>AFQETNPPAGPVRAIAEYERSAAVLVRYPFGIPMELIKELAKNDKVITIVASESQKNTVITQYTQSGVNLSNCDFIIAKTDSYWTRDYTGWFAMYDTNKVGLVDFIYNRPRPNDDEFPKYEAQYLGIEMFGMKLKQTGGNYMTDGYGSAVQSHIAYTENSSLSQAQVNQKMKDYLGITHHDVVQDPNNTYIDHVDCWGKYLAPNKILIRKVPDNHPQHQALEDMAAYFAAQTCAWGTKYEVYRALATNEQPYTNSLILNNRVFVPVNGPASVDNDALNVYKTAMPGYEIIGVKGASGTPWLGTDALHCRTHEVADKGYLYIK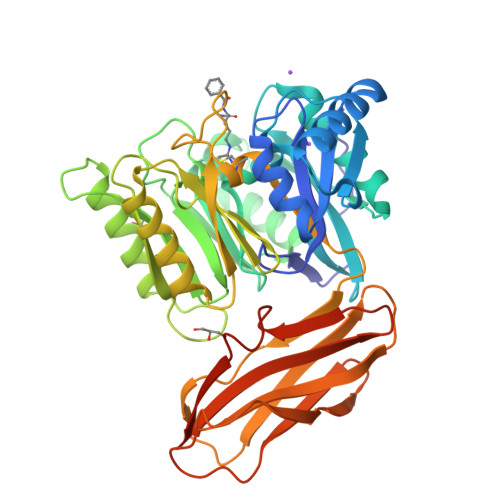HYPILGEQAGPDYKIEADVVSCANATISPVQCYYRINGSGSFKAADMTMESTGHYTYSFTGLNKNDKVEYYISAADNSGRKETYPFIGEPDPFKFTCMNETNTCTVTGAAHHHHHH[2x]McrBC is a two-component MDRS that in Escherichia coli (Ec) restricts phage DNA and foreign DNA containing methylated cytosines. EcMcrB consists of an N-terminal DNA-binding domain that targets fully or hemi-methylated RMC sites (where R is a purine base and MC is a 4-methyl-, 5-methyl-, or 5-hydroxymethyl-cytosine), and a C-terminal AAA+ (extended ATPases Associated with various cellular Activities) domain that hydrolyzes GTP and oligomerizes into hexamers. Biochemical data suggest that stimulated GTP hydrolysis powers DNA translocation, allowing EcMcrBC complexes bound to distant RMC sites to interact and induce cleavage on both strands. Here, we present cryo-EM structures of an McrB hexamer and McrBC complexes from the evolutionarily distant archaeal species Thermococcus gammatolerans (Tg) and the well-characterized E. coli system.

Purified TgMcrC was very sensitive to buffer conditions and could only be concentrated in the presence of TgMcrB. Together full-length TgMcrB and TgMcrC formed stable, dumbbell-shaped complexes in the presence of GTPγS that were suitable for structure determination by cryo-EM. Because of structural variability, however, we were only able to refine a “half”-complex, which yielded a map at an overall resolution of 2.4 Å. In this reconstruction, a single TgMcrC binds the TgMcrB hexamer by inserting itself through the central pore of the AAA+ ring in an asymmetric fashion. TgMcrC binding breaks the parallel π-stacking interaction between Arg414F and Tyr530E at the E/F interface, which has the smallest interaction area among the four tight interfaces (~2400 Å2 versus >2500 Å2 for all the others). Here, the helical bundle wedges against the D/E interface and inserts a highly conserved arginine (Arg263McrC) at the edge of the pocket. Acting through a hydrogen-bonding network that includes Asn359McrB, Asn410McrB, Asp413McrB, and a bridging water (H20Bridge), Arg263McrC ultimately alters the conformation of the McrB consensus loop. This reorganization allows Asn410 and E357 of the Walker B motif to position a second water (H20Cat) that is poised for nucleophilic attack on the γ-phosphate. The tight D/E interface shows an McrC-activated conformation with Arg426trans stabilizing the γ-phosphate and Asn410 properly arranged to orient the catalytic water. The loose F/A interface uniquely contains GDP with the side-chain oxygen of Asn410 forming a hydrogen bond with the β-phosphate. Our cryo-EM reconstruction of TgMcrBC unambiguously reveals the catalytic water molecules and illustrates how McrC’s insertion of a basic residue specifically repositions the signature motif to trigger hydrolysis, providing a chemically and energetically favorable description of stimulated turnover.

>[6x]MENQLFIIGIGTGTDEYENFEETILKGVKRNELEGQIGPDILDNCCSDVCYFWGRSKETIYEKKIDKGDMVLFYVGKRISRNKVDLNQETAVYLGIICETVEISENDVSFLNDFWRKGENFRFLMFFKKKPEKLHHSINEINSKLGYNPDYFPIAGYVKPERMSGVYDILKNILKKRGILKESDSMNESAGHNIKEDYFRVDMLLNKKGQVILYGPPGTGKTWIARKYVVEETNEKTPGNKWEFITFHQSYSYEEFIEGFRPRTDNEEKIRYVVEDGIFKKIALRALVKGLFELEDATIGKDKIHRLYILLTKKEPLSPTEYEEYLRLKRYLWELVGGLPKDKLKNLTPKFYLIIDEINRGNISKIFGELITLLEKDKRLGGENQLIVRLPYSGEPFAVPPNLYIIGTMNTADRSIALLDVALRRRFAFIEVEPRPEFLEKENLKKIREKKLKTEDRKRLNEKLNELFSKLGNDNYFLKTLLEKINVRITVVKDRDHRIGHSYFLNVETVEDLHHVWYYEVLPLLMEYFYNDWETIKWVLNEKGKEHGNVFFEKLRLTGPNGEEAYQLKVLEGDAFIGALKRIISKNTPSQEGGATTNEENSPENTQSQTEGD;> MPRLTTITLYEHDEKRYRDIAGDKKAIQDALIKLNKQFKKDFKKLDRSEDNSDTEDTIDESKGVVEVYANKIKARHYVGFAAVDNVFLQILPKVFKPKKEQTQETQEDTWEPILAFIRMLDMAYGLKIKDHDLAYLQGRNLRPNLYEVFIYLFAKSLWSEVQRGYHREYVEVHREEKFLRGKLLMSRQIRKLPHQLNTFSVEVHELIEDNLLNRIFYASVREALRRTTWGLNRKLLGELMLAFDGITPIHLRTEHFERVHFTRLNERFRRPFELAKLLFMPASGKGRSREVSGFFVDMNKLFERFIERVLVRNLPPEYKLFYQESYPFLKNQNGSSQKPDYVVRKGNTPVVVLDAKYRELKERIPSSDMLRQLYVYSRIWGYKTSHENDSKPPAVIVIPSSSTYNQGLPDKPLEFEFFDERKLFIVAYNMDYVKTGAIFKADKNFRRSLNNIIGKLNT The RGD (Arg-Gly-Asp)-binding integrins αvβ6 and αvβ8 are clinically validated cancer and fibrosis targets of considerable therapeutic importance. The highly homologous integrins αvβ6 and αvβ8 bind to latent transforming growth factor-β1 and β3 (L-TGF-β1 and L-TGF-β3) leading to release of active TGF-β1 and -β31–3. Here, we describe a method for computationally designing hyperstable RGD-containing miniproteins that are highly selective for a single RGD integrin heterodimer and conformational state, and use this strategy to design inhibitors of αvβ6 and αvβ8 with high selectivity. We found small α/β ferredoxin folds were able to scaffold the RGDLXX(L/I) binding loop without clashing with the integrin while making additional contacts with both α and β subunit (α- and β-loop respectively).

Following two rounds of design and optimization (see supplementary info for details), two high affinity variants were selected for further characterization: B6B8_BP (av6_3_E13T) and B6_BP (av6_3_A39KG64R). Affinity maturation identified a substitution to a lysine (A39K) making a salt-bridge interaction with E316 of the β6 subunit while the LXX(L/I) motif remained fixed confirming the importance of this motif for selectivity towards αvβ6. In B6_BP, the β-loop is positioned to confer selectivity between the two integrins, where residue K39 faces E316 on the β6 subunit and K304 on β8. B6_BP binds αvβ6 with a higher affinity than αvβ8 on the surface of K562 cells, with a Kd of 0.11 (±0.09) and 580 (±40) nM, respectively. As intended, B6_BP is more selective for αvβ6 than B6B8_BP. B6B8_BP and B6_BP do not cross-react with RGD-binding integrins αvβ1, αvβ3, αvβ5, α5β1, α8β1, and αiibβ3 at concentrations up to 200 nM in cell surface binding experiments using K562 cells stably transfected with different RGD-binding integrins, corresponding to >1000-fold selectivity. As B6_BP binds to A431 cells with higher affinity and is more selective than B6B8_BP for αvβ6, we selected B6_BP for further in vivo experiments. AF680-B6_BP rapidly accumulated in the αvβ6 positive tumors and reached a high tumor-to-muscle fluorescence contrast ratio within 3 h post-injection.

>AVVRFVFRGDLAELMLRAVKDHLKKEGPHWNITSRGNELVVRGIHESDAKRIQKEFPSVQSTIQAAAAAA[12x]>MKDLVDTTEMYLRTIYELEEEGVTPLRARIAERLEQSGPTVSQTVARMERDGLVVVASDRSLQMTPTGRTLATAVMRKHRLAERLLTDIIGLDINKVHDEADRWEHVMS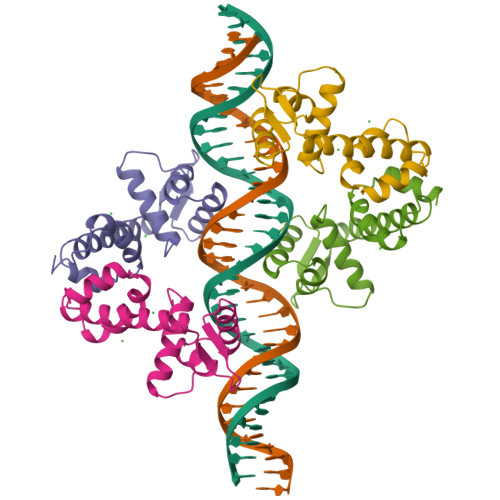DEVERRLVKVLKDVSRSPFGNPIPGLDELGVGNSDAAAPGTRVIDAATSMPRKVRIVQINEIFQVETDQFTQLLDADIRVGSEVEIVDRDGHITLSHNGKDVELLDDLAHTIRIEEL[4x]>[8x]MKTSDANETEDHLESLICKVGEKSACSLESNLEGLAGVLEADLPNYKSKILRLLCTVARLLPEKLTIYTTLVGLLNARNYNFGGEFVEAMIRQLKESLKANNYNEAVYLVRFLSDLVNCHVIAAPSMVAMFENFVSVTQEEDVPQVRRDWYVYAFLSSLPWVGKELYEKKDAEMDRIFANTESYLKRRQKTHVPMLQVWTADKPHPQEEYLDCLWAQIQKLKKDRWQE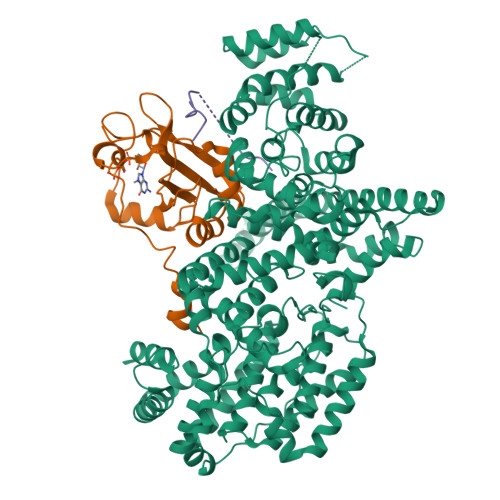RHILRPYLAFDSILCEALQHNLPPFTPPPHTEDSVYPMPRVIFRMFDYTDDPEGPVMPGSHSVERFVIEENLHCIIKSHWKERKTCAAQLVSYPGKNKIPLNYHIVEVIFAELFQLPAPPHIDVMYTTLLIELCKLQPGSLPQVLAQATEMLYMRLDTMNTTCVDRFINWFSHHLSNFQFRWSWEDWSDCLSQDPESPKPKFVREVLEKCMRLSYHQRILDIVPPTFSALCPVNPTCIYKYGDESSNSLPGHSVALCLAVAFKSKATNDEIFSILKDVPNPNQDDDDDEGFSFNPLKIEVFVQTLLHLAAKSFSHSFSALAKFHEVFKTLAESDEGKLHVLRVMFEVWRNHPQMIAVLVDKMIRTQIVDCAAVANWIFSSELSRDFTRLFVWEILHSTIRKMNKHVLKIQKELEEAKEKLARQHKRRSDDDDRSSDRKDGVLEEQIERLQEKVESAQSEQKNLFLVIFQRFIMILTEHLVRCETDGTSVLTPWYKNCIERLQQIFLQHHQIIQQYMVTLENLLFTAELDPHILAVFQQFCALQA;>[8x]GAMSGGLLKALRSDSYVELSQYRDQHFRGDNEEQEKLLKKSCTLYVGNLSFYTTEEQIYELFSKSGDIKKIIMGLDKMKKTACGFCFVEYYSRADAENAMRYINGTRLDDRIIRTDWDAGFKEGRQYGRGRSGGQVRDEYRQDYDAGRGGYGKLAQNQ;>GAMGRGNYDAFRGQGGYPGKPRNRMVRGDPRAIVEYRDLDAPDDVDFF[8x]While most SAM riboswitches strongly discriminate between SAM and SAH, the SAM/SAH riboswitch responds to both ligands with similar apparent affinities. The riboswitch forms an H-type pseudoknot structure with coaxial alignment of the stem–loop helix (P1) and the pseudoknot helix (PK). An additional three base pairs form at the non-open end of P1, and the ligand is bound at the interface between the P1 extension and the PK helix. Binding SAM or SAH stabilizes the PK helix, so structuring the Shine–Dalgarno sequence, sequestering it and preventing initiation of translation (OFF state).

All retain the adenosine moiety, with variations in the methionine chain attached to the 5′ position. The adenosine sections are bound identically in all six complexes, with the same four hydrogen bonds between the RNA and ligand in each case. The differences lie in the methionine section of the molecules. The specificity of binding is largely realized through the adenosine moiety, forming four hydrogen bonds to the riboswitch RNA in each case.

>[6x]GGUCACAACGGCUUCCUGGCGUGACC;>AUUGGAGCA[6x]> RDITRRLKSIKNIQKITKSMKMVAAAKYARAERELKPARVYGTGSLALYEKAEIKGPEDKKKHLIIGVSSDRGLCGAIHSSVAKQMKNDMAALTAAGKEVMIVGIGEKIKSILYRTHSDQFLVSFKDVGRKPPTFGDASVIALELLNSGYEFDEGSIIFNQFKSVISYKTEEKPIFSFSTVVAAENMSIYDDIDADVLQNYQEYNLANIIYYSLKESTTSEQSARMTAMDNASKNASDMIDKLTLTFNRTRQAVITKELIEIISGAAAL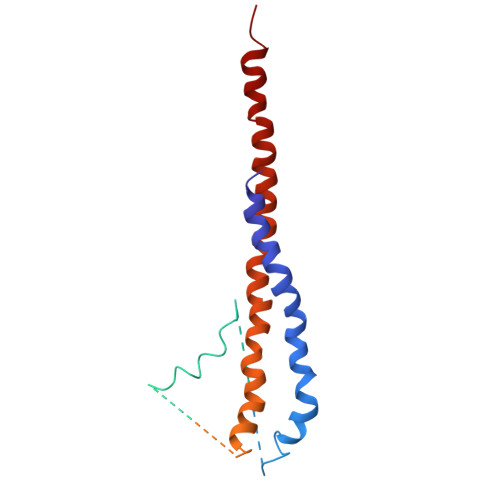D>MGSSHHHHHHSQDPAVPYNRMKLMIVGNTGSGKTTLLQQLMKTKKSDLGMQSATVGIDVKDWPIQIRDKRKRDLVLNVWDFAGREEFYSTHPHFMTQRALYLAVYDLSKGQAEVDAMKPWLFNIKARASSSPVILVGTHLDVSDEKQRKACMSKITKELLNKRGFPAIRDYHFVNATEESDALAKLRKTIINESLNFK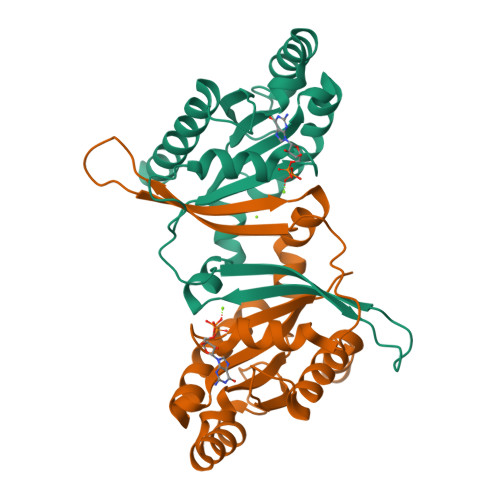IRDQLVVG[2x]>[2x]GMQGAGRLMQPRP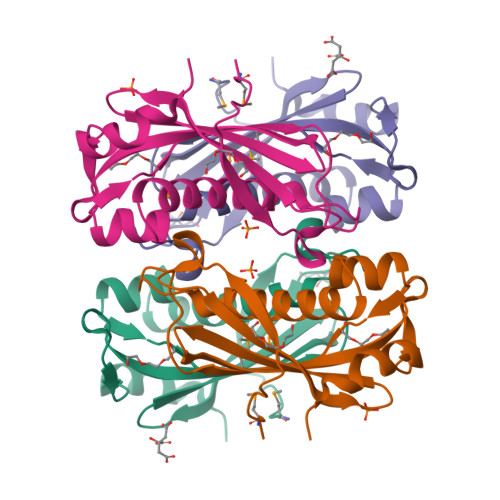DSAFVHDVRVTWGDCDPAKIAYTGHLPRFALEAIDAWWSEYHGPGGWYHLELDTNVGTPFVRLEMDFKSPVTPRHILKCHTWPTRLGTKSITFRVDGVQDGVTCFVGAFTCVFTIADQFKSQPAPDHLRALIEPHIPA>MKIFLDTANIDEIRTGVNWGIVDGVTTNPDLISKEAVNGKKYGDIIREILKIVDGPVSVEVVSTKYEGMVEEARKIHGLGDNAVVKIPMTEDGLRAIKTLSSEHINTNCTLVFNPIQALLAAKAGVTYVSPFVGRLDDIGEDGMQIIDMIRTIFNNYIIKTQILVASIRNPIHVLRSAVIGADVVTVPFNVLKSLMKHPKTDEGLAKFLE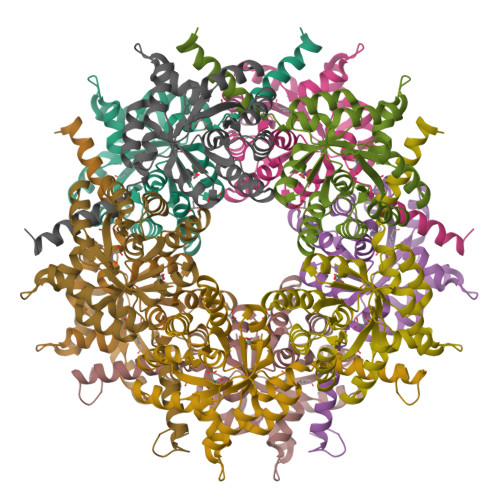DWKKVSPDGKLIL[5x]> NTGRTEAWK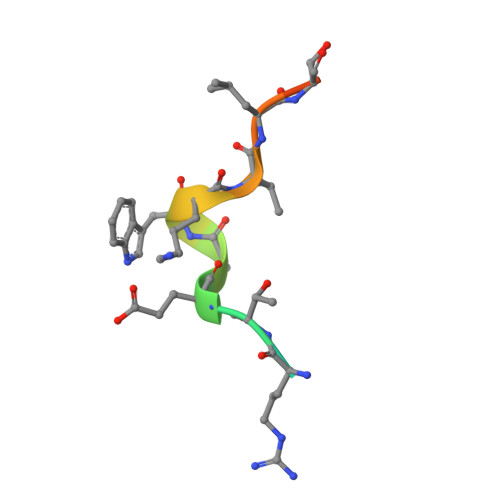VLSPQG> TIVKSEIIRKLMDAKKFLLDGYIDEGVKIVLEITKSSTKSEYNWFICNLLESIDCRYMFQVLDKIGSYFDLDKCQNLKSVVECGVINNTLNEHVNKALDILVIQGKRDKLEEIGREILK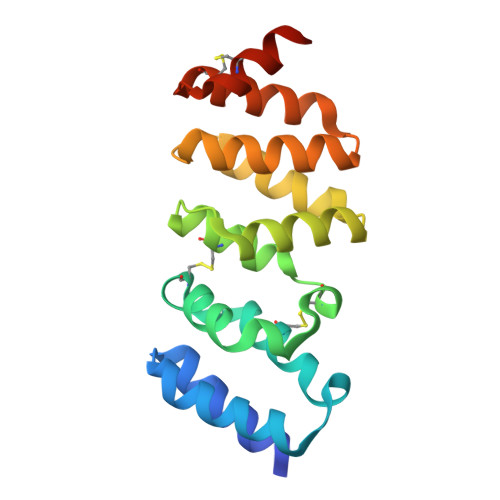NNEVSASILVAIANALRRVGDERDATTLLIEACKKGEKEACNAVNTLTVRSVM>GSSRGFPEDSEPISISHGNYTKQYPVFVGHKPGRNTTQRHRLDIQMIMIMNRTLYVAARDHIYTVDIDTSHTEEIYCSKKLTWKSRQADVDTCRMKGKHKDECHNFIKVLLKKNDDTLFVCGTNAFNPSCRNYRVDTLETFGDEFSGMARCPYDAKHANIALFADGKLYSATVTDFLAIDAVIYRSLGDSPTLRTVKHDSKWLKEPYFVQAVDYGDYIYFFFREIAVEYNTMGKVVFPRVAQVCKNDMGGSQRVLEKQWTSFLKARLNCSVPGDSHFYFNILQAVTDVIRINGRDVVLATFSTPYNSIPGSAVCAYDMLDIANVFTGRFKEQKSPDSTWTPVPDERVPKPRPGCCAGSSSLEKYATSNEFPDDTLNFIKTHPLMDEAVPSIINRPWFLRTMVRYRLTKIAVDNAAGPYQNHTVVFLGSEKGIILKFLARIGSSGFLNGSLFLEEMNVYNPEKCSYDGV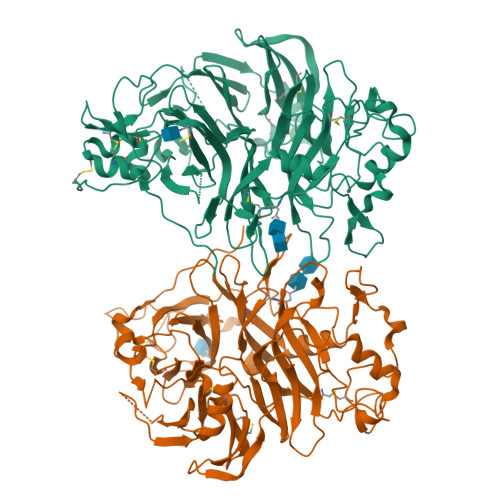EDKRIMGMQLDRASGSLYVAFSTCVIKVPLGRCERHGKCKKTCIASRDPYCGWVRESGSCAHLSPLSRLTFEQDIERGNTDGLGDCHN[2x]> MGKEKSHINVVVIGHVDSGKSTT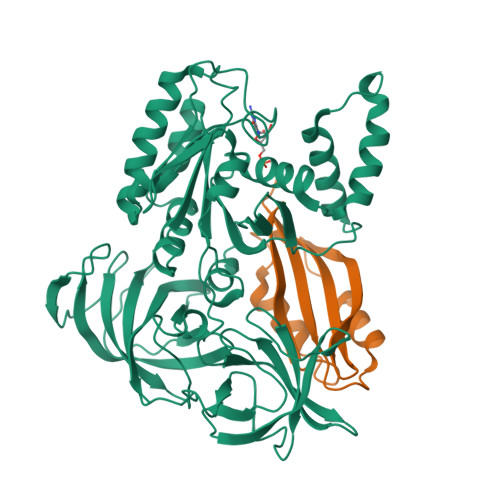TGHLIYKCGGIDKRTIEKFEKEAAELGKGSFKYAWVLDKLKAERERGITIDIALWKFETPKYQVTVIDAPGHRDFIKNMITGTSQADCAILIIAGGVGEFEAGISKDGQTREHALLAFTLGVRQLIVAVNKMDSVKWDESRFQEIVKETSNFIKKVGYNPKTVPFVPISGWNGDNMIEATTNAPWYKGWEKETKAGVVKGKTLLEAIDAIEQPSRPTDKPLRLPLQDVYKIGGIGTVPVGRVETGVIKPGMVVTFAPAGVTTEVKSVEMHHEQLEQGVPGDNVGFNVKNVSVKEIRRGNVCGDAKNDPPKGCASFNATVIVLNHPGQISAGYSPVLDCHTAHIACRFDELLEKNDRRSGKKLEDHPKFLKSGDAALVKFVPSKPMCVEAFSEYPPLGRFAVRDMRQTVAVGVIKSVDKTEKAAKVTKAAQKAAKK;> PAAKSIVTLDVKPWDDETNLEEMVANVKAIEMEGLTWGAHQFIPIGFGIKKLQINCVVEDDKVSLDDLQQSIEEDEDHVQSTDIAAMQKL>AELPQMVQQLNSPDQQELQSALRKLSQIASGGNEQIQAVIDAGALPALVQLLSSPNEQILQEALWTLGNIASGGNEQIQAVIDAGALPALVQLLSSPNEQ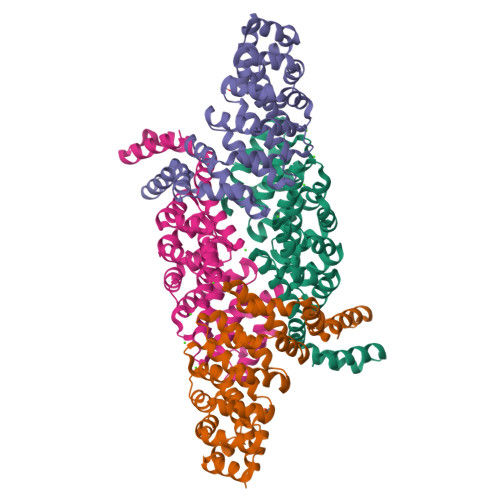ILQEALWTLGNIASGGNEQIQAVIDAGALPALVQLLSSPNEQILQEALWTLGNIASGGNEQIQAVIDAGALPALVQLLSSPNEQILQEALWTLGNIASGGNEQIQAVIDAGALPALVQLLSSPNEQILQEALWTLGNIASGGNEQKQAVKEAGAEPALEQLQSSPNEKIQKEAQEALEKIQ[4x]> MTSTLTWPLRIAWFLLWFFWQQTTTSAKVVRDAFLPHASITPGFVRFPTRCRSEL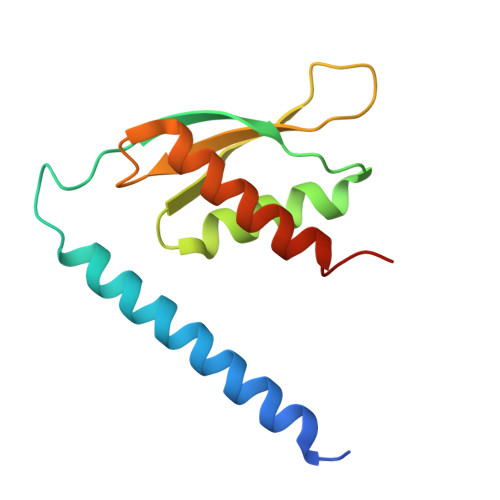EVTMLSSLITLTPGTLTLGAHHPGEGEDWEIVVHGMYFPDPDDLTASLHDLENHMLRAIRREGLTR> MRHERVVIIKNMFHPMDFED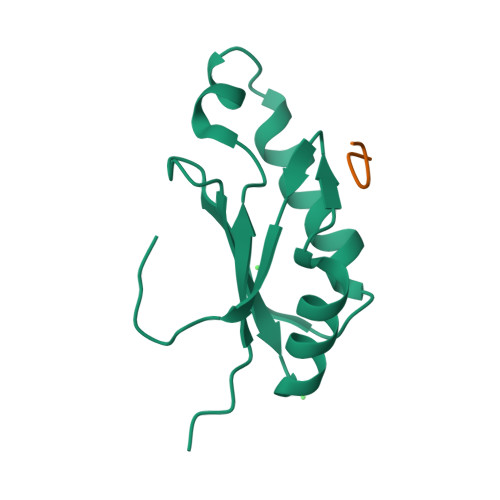DPLVLNEIREDLRVECSKFGQIRKLLLFDRHPDGVASVSFRDPEEADYCIQTLDGRWFGGRQITAQAWDGTTDY;> SRWDVK> MAMHPRKDWYELTRATNWTPSYVTEEQLFPERMSGHMGIPLEKWESYDEPYKTSYPEYVSIQREKDAGAYSVKAALERAKIYENSDPGWISTLKSHYGAIAVGEYAAVTGEGRMARFSKAPGNRNMATFGMMDELRHGQLQLFFPHEYCKKDRQFDWAWRAYHSNEWAAIAAKHFFDDIITGRDAISVAIMLTFSFETGFANMQFLGLAADAAEAGDYTFANLISSIQTDESRHAQQGGPALQLLIENGKREEAQKKVDMAIWRAWRLFAVLTGPVMDYYTPLEDRSQSFKEFMYEWIIGQFERSLIDLGLDKPWYWDLFLKDIDELHHSYHMGVWYWRTTAWWNPAAGVTPEERDWLEEKYPGWNKRWGRCWDVITENVLNDRMDLVSPETLPSVCNMSQIPLVGVPGDDWNIEVFSLEHNGRLYHFGSEVDRWVFQQDPVQYQNHMNIVDRFLAGQIQPMTLEGALKYMGFQSIEEMGKDAHDFAWADKCKPAMKKSA;> MSFESKKPMRTWSHLAEMRKKPSEYDIVSRKLHYSTNNPDSPWELSPDSPMNLWYKQYRNASPLKHDNWDAFTDPDQLVYRTYNLMQDGQESYVQSLFDQFNEREHDQMVREGWEHTMARCYSPLRYLFHCLQMSSAYVQQMAPASTISNCCILQTADSLRWLTHTAYRTHELSLTYPDAGLGEHERELWEKEPGWQGLRELMEKQLTAFDWGEAFVSLNLVVKPMIVESIFKPLQQQAWENNDTLLPLLIDSQLKDAERHSRWSKALVKHALENPDNHAVIEGWIEKWRPLADRAAEAYLSMLSSDILHAQYLERS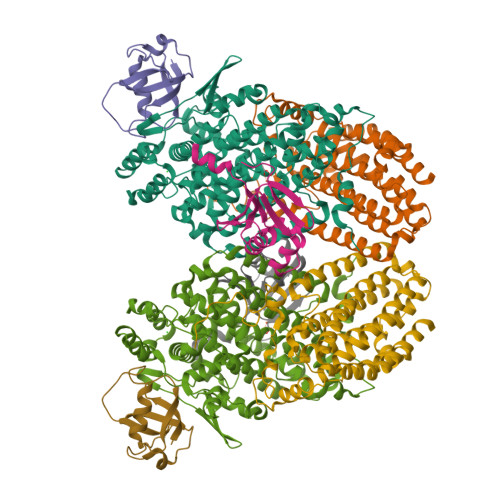TSLRASILTV;> MSAFPVHAAFEKDFLVQLVVVDLNDSMDQVAEKVAYHCVNRRVAPREGVMRVRKHRSTELFPRDMTIAESGLNPTEVIDVVFEE;> MSTLADQALHNNNVGPIIRAGDLVEPVIETAEIDNPGKEITVEDRRAYVRIAAEGELILTRKTLEEQLGRPFNMQELEINLASFAGQIQADEDQIRFYFDKTM>[2x]GSHMASSHLAELVASAKAAISQASDVAALDNVRVEYLGKKGHLTLQMTTLRELPPEERPAAGAVINEAKEQVQQALNARKAELESAALNARLAAETIDVSLPGRRIENGGLHPVTRTIDRIESFFGELGFTVATGPEIEDDYHNFDALNIPGHHPARADHDTFWFDTTRLLRTQTSGVQIRTMKAQQPPIRIIAPGRVYRNDYDQTHTPMFHQMEGLIVDTNISFTNLKGTLHDFLRNFFEEDLQIRFRPSYFPFTEPSAEVDVMGKNGKWLEVLGCGMVHPNVLRNVGIDPEVYSGFAFGMGMERLTMLRYGVTDLRSFFENDLRFLKQFK;>[2x]MKFSELWLREWVNPAIDSDALANQITMAGLEVDGVEPVAGSFHGVVVGEVVECAQHPNADKLRVTKVNVGGDRLLDIVCGAPNCRQGLRVAVATIGAVLPGDFKIKAAKLRGEPSEGMLCSFSELGISDDHSGIIELPADAPIGTDIREYLKLDDNTIEISVTPNRADCLGIIGVARDVAVLNQLPLVQPEIVPVGATIDDTLPITVEAPEACPRYLGRVVKGINVKAPTPLWMKEKLRRCGIRSIDAVVDVTNYVLLELGQPMHAFDKDRIEGGIVVRMAKEGETLVLLDGTEAKLNADTLVIADHNKALAMGGIFGGEHSGVNDETQNVLLECAFFSPLSITGRARRHGLHTDASHRYERGVDPALQHKAMERATRLLIDICGGEAGPVIDITNEATLPKRATITLRRS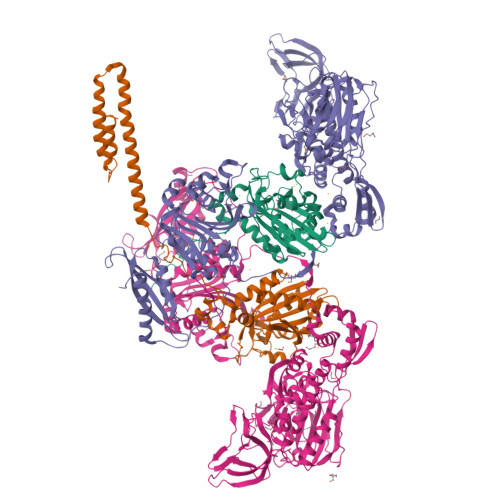KLDRLIGHHIADEQVTDILRRLGCEVTEGKDEWQAVAPSWRFDMEIEEDLVEEVARVYGYNNIPDEPVQASLIMGTHREADLSLKRVKTLLNDKGYQEVITYSFVDPKVQQMIHPGVEALLLPSPISVEMSAMRLSLWTGLLATVVYNQNRQQNRVRIFESGLRFVPDTQAPLGIRQDLMLAGVICGNRYEEHWNLAKETVDFYDLKGDLESVLDLTGKLNEVEFRAEANPALHPGQSAAIYLKGERIGFVGVVHPELERKLDLNGRTLVFELEWNKLADRVVPQAREISRFPANRRDIAVVVAENVPAADILSECKKVGVNQVVGVNLFDVYRGKGVAEGYKSLAISLILQDTSRTLEEEEIAATVAKCVEALKERFQASLRD Kustd1711 is a putative electron transfer protein encoded on the nitrite oxidoreductase (nxr) gene cluster of anaerobic ammonium-oxidizing (anammox) bacteria and consists of two heme-containing domains and one additional domain. Here, we describe a diheme cytochrome c with high heme redox potentials of about +350 mV, despite having a large overall negative charge, which typically reduces redox potentials. High-resolution crystal structures, spectroelectrochemical measurements, and high-end computational methods show how this is achieved: each heme iron has a calcium cation positioned next to it at a distance of only 6.9 Å, raising their redox potentials by several hundred millivolts through electrostatic interaction. We suggest that this has evolved to provide the protein with a high redox potential despite its large negative surface charge, which it likely requires for interactions with redox partners.

To improve our confidence in the assignment of the various transitions, we mutated the distal methionine ligands in both the N- and C-terminal heme sites to histidine and cysteine. To confirm that the sites can accommodate these mutations while maintaining six-coordinate heme binding and calcium binding, we determined the crystal structures of the C-terminal domain methionine mutants M292H and M292C to 1.12 and 1.70 Å resolution, respectively using the same crystallization conditions as for the wt protein, that is, including 200 mM Ca2+. This showed that these mutants are able to support both six-coordinate heme ligation as well as calcium binding, although in the M292H mutant, the plane of the distal His292’s side chain is at an angle of ∼75° with the plane of the heme porphyrin system rather than perpendicular to it. The M→H mutants, however, yielded data with clear transitions and little hysteresis. As the mutation of a distal methionine to histidine in a c-type cytochrome typically results in a drop in redox potential of ∼320 mV, in each mutant, one of the two transitions in each of the two pairs can be expected to drop by approximately this amount. In addition, mutations of either of the heme sites’ distal heme-coordinating methionine to histidine change the relative amplitudes of the various transitions. To at least some extent, this could be explained by changes in extinction coefficients caused by the mutation. However, it is also possible that these mutations have compromised calcium binding. That the crystal structures of the mutant showed a fully occupied calcium site in both domains is probably because of the high (200 mM) calcium concentration used in crystallization.

> MNKTMLKIVAFGVAVIGFYMYITVYVTGLSGTGGGGTATGVSAEAGEQIFWGDGQCSTCHKIGSSGSATRGPDQEGLAERAEERAKELGLSSGLEYLVESIIDPEKYVVEGFDKIMPRVYDPPIMLSREKILAVLAYLQSLGGEPDLDAIMKFKDKIPEASKTKVKPWVPPLAVTAEEGEQVFFDESLDVTCGKCHMVNGKGQKVGPELTGIGAIQTPQYFVESILEPSAVIVKGYETVFVITADGIPYNGLIKSDTEEELTLILEESGSVEEVVIPKDEIEDMKKQEVSIHPGNIGELLSVRQFYAVIEYLRSLK>MANGVIPPPGGASPLPQVRVPLEEPPLSPDVEEEDDDLGKTLAVSRFGDLISKPPAWDPEKPSRSYSERDFEFHRHTSHHTHHPLSARLPPPHKLRRLPPTSARHTRRKRKKEKTSAPPSEGTPPIQEEGGAGVDEEEEEEEEEEGESEAEPVEPPHSGTPQKAKFSIGSDEDDSPGLPGRAAVTKPLPSVGPHTDKSPQHSSSSPSPRARASRLAGEKSRPWSPSASYDLRERLCPGSALGNPGGPEQQVPTDEAEAQMLGSADLDDMKSHRLEDNPGVRRHLVKKPSRTQGGRGSPSGLAPILRRKKKKKKLDRRPHEVFVELNELMLDRSQEPHWRETARWIKFEEDVEEETERWGKPHVASLSFRSLLELRRTIAHGAALLDLEQTTLPGIAHLVVETMIVSDQIRPEDRASVLRTLLLKHSHPNDDKDSGFFPRNPSS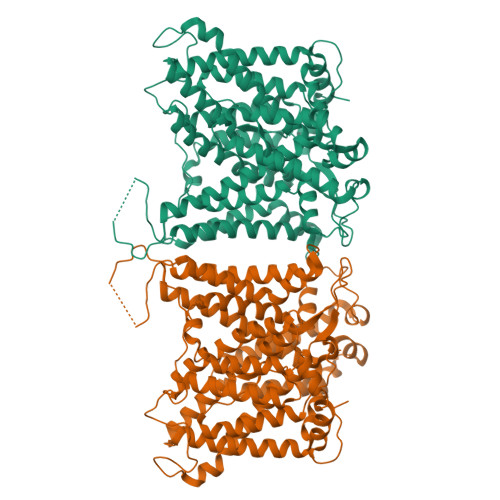SSMNSVLGNHHPTPSHGPDGAVPTMADDLGEPAPLWPHDPDAKEKPLHMPGGDGHRGKSLKLLEKIPEDAEATVVLVGCVPFLEQPAAAFVRLNEAVLLESVLEVPVPVRFLFVMLGPSHTSTDYHELGRSIATLMSDKLFHEAAYQADDRQDLLSAISEFLDGSIVIPPSEVEGRDLLRSVAAFQRELLRKRREREQTKVEMTTRGGYTAPGKELSLELGGSEATPEDDPLLRTGSVFGGLVRDVRRRYPHYPSDLRDALHSQCVAAVLFIYFAALSPAITFGGLLGEKTEGLMGVSELIVSTAVLGVLFSLLGAQPLLVVGFSGPLLVFEEAFFKFCRAQDLEYLTGRVWVGLWLVVFVLALVAAEGSFLVRYISPFTQEIFAFLISLIFIYETFYKLYKVFTEHPLLPFYPPEGALEGSLDAGLEPNGSALPPTEGPPSPRNQPNTALLSLILMLGTFFIAFFLRKFRNSRFLGGKARRIIGDFGIPISILVMVLVDYSITDTYTQKLTVPTGLSVTSPDKRSWFIPPLGSARPFPPWMMVAAAVPALLVLILIFMETQITALIVSQKARRLLKGSGFHLDLLLIGSLGGLCGLFGLPWLTAATVRSVTHVNALTVMRTAIAPGDKPQIQEVREQRVTGVLIASLVGLSIVMGAVLRRIPLAVLFGIFLYMGVTSLSGIQLSQRLLLILMPAKHHPEQPYVTKVKTWRMHLFTCIQLGCIALLWVVKSTAASLAFPFLLLLTVPLRHCLLPRLFQDRELQALDSEDAEPNFDEDGQDEYNELHMPV[2x]> TEMSVRKIAAHMKSNPNAKVIFMVGAGISTSCGIPDFRSPGTGLYHNLARLKLPYPEAVFDVDFFQSDPLPFYTLAKELYPGNFRPSKFHYLLKLFQDKDVLKRVYTQNIDTLERQAGVKDDLIIEAHGSFAHCHCIGCGKVYPPQVFKSKLAEHPIKDFVKCDVCGELVKPAIVFFGEDLPDSFSETWLNDSEWLREKITTSGKHPQQPLVIVVGTSLAVYPFASLPEEIPRKVKRVLCNLETVGDFKANKRPTDLIVHQYSDEFAEQLVEELGWQEDFEKILTAQ;> QTARKSTGGK

Lysine benzoylation (Kbz) is a recently discovered post-translational modification associated with active transcription. Here, we systematically characterize writer, eraser, and reader proteins of histone Kbz in S. cerevisiae using proteomic, biochemical, and structural approaches. The Spt-Ada-Gcn5 acetyltransferase (SAGA) complex and NAD+-dependent histone deacetylase Hst2 could function as the writer and eraser of histone Kbz, respectively. In addition, we demonstrate that a subset of YEATS domains and bromodomains serve as Kbz readers, and structural analyses reveal how YEATS and bromodomains recognize Kbz marks.

To elucidate the molecular mechanism of Hst2-mediated debenzoylation, we determined the crystal structure of Hst28-294 in the complex with the benzoylated H3 peptide (H35-14K9bz) at 2.0 Å resolution. In both structures, Hst28-294 exhibits an elongated structure containing a large Rossmann-fold domain and a small zinc-containing domain. The small domain consists of four α-helices (α3-5, α9) and three β-strands (β4-6). Both the H3 peptide and the cofactor product bind to the cleft between two domains. In the Hst2-peptide structure, histone H3 residues from T6 to K14 were modeled based on the electron density. The histone peptide adopts a bent conformation and makes extensive contacts with Hst2 through both electrostatic and hydrophobic interaction. The majority of H3 binds to a negatively charged surface of Hst2, explaining the preference of benzoylated lysine flanked by positively charged residues. Specifically, H3 R8 is positioned in an acidic patch containing Hst2 D68 and D70, reinforcing the notion that the strong histone binders of Hst2 (H3K9, H3K18, and H3K27) share the RK signature. Benzoylated lysine 9 (K9bz) is snugly inserted into a relatively hydrophobic tunnel and adopts the same geometric configuration of H4K16ac as seen in the Hst2-H4K16ac structure. The bulky benzene ring of K9bz induces a 20° rotation of the phenyl group of F67 to coordinate a π-π stacking interaction with the benzene ring. Additionally, K9bz induces shifts of I117 and I181 to generate a larger space to accommodate the benzene ring.> MVPGSEGPARAGSVVADVVFVIEGTANLGPYFEGLRKHYLLPAIEYFNGGPPAETDFGGDYGGTQYSLVVFNTVDCAPESYVQCHAPTSSAYEFVTWLDGIKFMGGGGESCSLIAEGLSTALQLFDDFKKMREQIGQTHRVCLLICNSPPYLLPAVESTTYSGCTTENLVQQIGERGIHFSIVSPRKLPALRLLFEKAAPPALLEPLQPPTDVSQDPRHMVLVRGLVLPVGGGSAPGPLQSKQPVPLPPAAPSGATLSAAPQQPLPPVPPQYQVPGNLSAAQVAAQNAVEAAKNQKAGLGPRFSPITPLQQAAPGVGPPFSQAPAPQLPPGPPGAPKPPPASQPSLVSTVAPGSGLAPTAQPGAPSMAGTVAPGGVSGPSPAQLGAPALGGQQSVSNKLLAWSGVLEWQEKPKPASVDANTKLTRSLPCQVYVNHGENLKTEQWPQKLIMQLIPQQLLTTLGPLFRNSRMVQFHFTNKDLESLKGLYRIMGNGFAGCVHFPHTAPCEVRVLML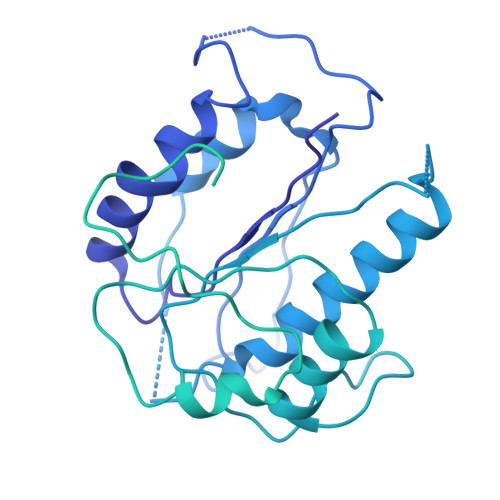LYSSKKKIFMGLIPYDQSGFVNGIRQVITNHKQVQQQKLEQQQRGMGGQQAPPGLGPILEDQARPSQNLLQLRPPQPQPQGTVGASGATGQPQPQGTAQPPPGAPQGPPGAASGPPPPGPILRPQNPGANPQLRSLLLNPPPPQTGVPPPQASLHHLQPPGAPALLPPPHQGLGQPQLGPPLLHPPPAQSWPAQLPPRAPLPGQMLLSGGPRGPVPQPGLQPSVMEDDILMDLI>[8x]MNTDVRIEKDFLGEKEIPKDAYYGVQTIRATENFPITGYRIHPELIKSLGIVKKSAALANMEVGLLDKEVGQYIVKAADEVIEGKWNDQFIVDPIQGGA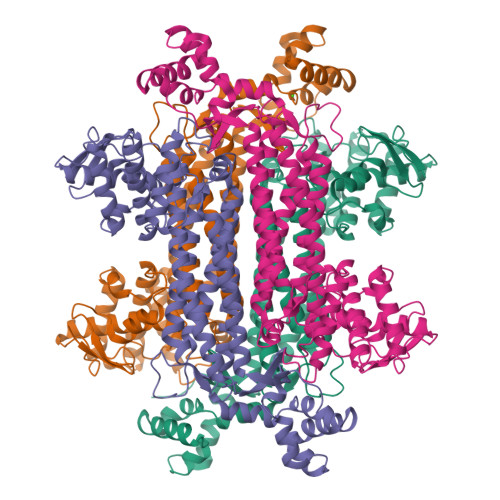GTSINMNANEVIANRALELMGEEKGNYSKISPNSHVNMSQSTNDAFPTATHIAVLSLLNQLIETTKYMQQEFMKKADEFAGVIKMGRTHLQDAVPILLGQEFEAYARVIARDIERIANTRNNLYDINMGATAVGTGLNADPEYISIVTEHLAKFSGHPLRSAQHLVDATQNTDCYTEVSSALKVCMINMSKIANDLRLMASGPRAGLSEIVLPARQPGSSIMPGKVNPVMPEVMNQVAFQVFGNDLTITSASEAGQFELNVMEPVLFFNLIQSISIMTNVFKSFTENCLKGIKANEERMKEYVEKSIGIITAINPHVGYETAAKLAREAYLTGESIRELCIKYGVLTEEQLNEILNPYEMIHPGIAGRK> MTNIEILENMLKLQQKLNDETNGLNWENGYTKEGKLISWRRCIYMECAELIDSFTWKHWKNISSLTNWENVRIEIVDIWHFILSLLLEEYRDKNNKDFKAIATEVNAVSVFQDFCKEEEYPNEGDIYGILNDIELIIHKCSGFGFNLGELLSTYF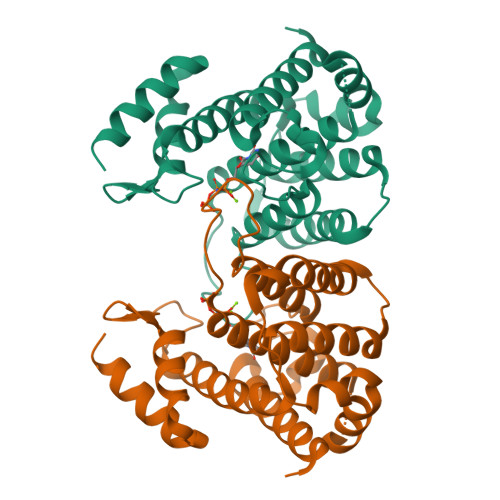TLAIKCGLNLEILYKTYIGKNVLNIFRQNNGYKDGSYKKTWNGKEDNEVLAQILEQELDFDTIYKKLEECYKKA>[2x]GSH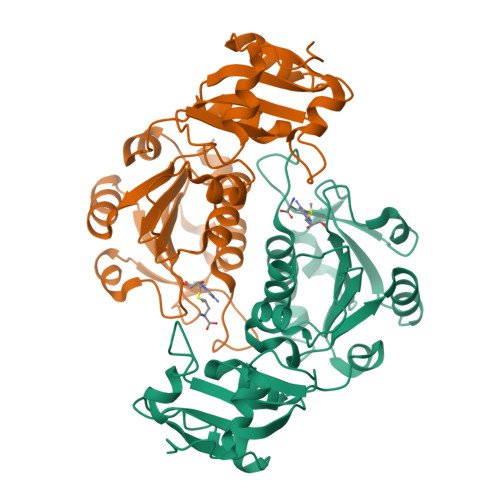MTELDTIANPSDPAVQRIIDVTKPSRSNIKTTLIEDVEPLMHSIAAGVEFIEVYGSDSSPFPSELLDLCGRQNIPVRLIDSSIVNQLFKGERKAKTFGIARVPRPARFGDIASRRGDVVVLDGVKIVGNIGAIVRTSLALGASGIILVDSDITSIADRRLQRASRGYVFSLPVVLSGREEAIAFIRDSGMQLMTLKADGDISVKELGDNPDRLALLFGSEKGGPSDLFEEASSASVSIPMMSQTESLNVSVSLGIALHERIDRNLAANR> MSTQYETQGYTINNAGRRLVVDPITRIEGHMRCEVNINDQNVITNAVSCGTMFRGLEIILQGRDPRDAWAFVERICGVCTGVHALASVYAIEDAIGIKVPDNANIIRNIMLATLWCHDHLVHFYQLAGMDWIDVLDALKADPRKTSELAQSLSSWPKSSPGYFFDVQNRLKKFVEGGQLGIFRNGYWGHPQYKLPPEANLMGFAHYLEALDFQREIVKIHAVFGGKNPHPNWIVGGMPCAINIDESGAVGAVNMERLNLVQSIITRTADFINNVMIPDALAIGQFNKPWSEIGTGLSDKCVLSYGAFPDIANDFGEKSLLMPGGAVINGDFNNVLPVDLVDPQQVQEFVDHAWYRYPNDQVGRHPFDG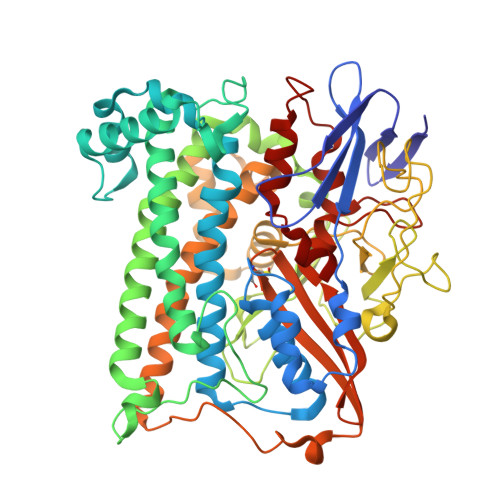ITDPWYNPGDVKGSDTNIQQLNEQERYSWIKAPRWRGNAMEVGPLARTLIAYHKGDAATVESVDRMMSALNLPLSGIQSTLGRILCRAHEAQWAAGKLQYFFDKLMTNLKNGNLATASTEKWEPATWPTECRGVGFTEAPRGALGHWAAIRDGKIDLYQCVVPTTWNASPRDPKGQIGAYEAALMNTKMAIPEQPLEILRTLHSFDPCLACSTH>[2x]MARQTMNPSIRYLIGVDGGGTGTRIRLHASDGTPLAMAEGGASALSQGIAKSWQAVLSTLEAAFQQAGLPAAPASACAIGLGLSGVHNRQWAGEFESQAPGFARLSLATDGYTTLLGAHGGQPGIIVALGTGSIGEALYPDGSHREAGGWGYPSGDEASGAWLGQRAAQLTQMALDGRHSHSPLTRAVLDFVGGDWQAMMAWNGRATPAQFARLAPLVLSAA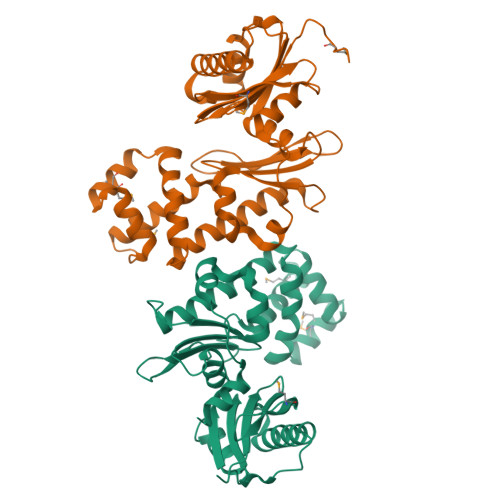RVDPEADALLRQAGEDAWAIARALDPQDELPVALCGGLGQALRDWLPPGFRQRLVAPQGDSAQGALLLLQRPSTRLEHHHHHH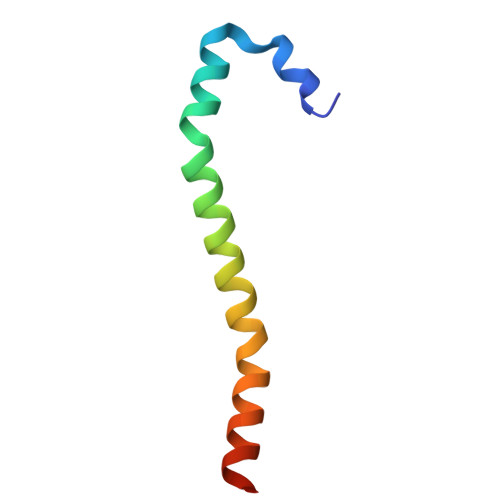> GEFEFLKFLTFDDLNQRLCNIDHEMELEIEQLNKKYNAKRQPIVDAMNAKRKRQQNI>[46x]MAKGRTPRSFSQRYGKWNAKFTAFSNPTVASTILTNVAPIAQGNFQTNVPKFTSVNEQVSAVLTQYGVTGPSRA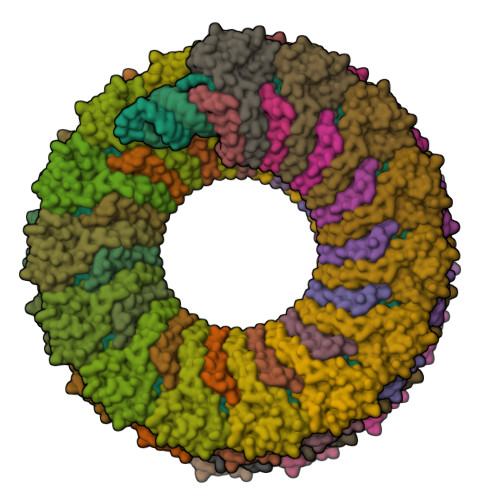IYQGYGLKVARALNRIGAGPALTNMVAGLKAYYVSAYGANPEILDAVTNIILGSPTGYVS> SGPLGSEAHLYMQVQIVAEDQFCGHQGNDMYDEEKVKYTVFKVLKNSSLAEFVQSLSQTMGFPQDQIRLWPMQARSNGTKRPAMLDNEADGNKTMIELSDNENPWTIFLETVDPELAASGATLPKFDKDHDVMLFLKMYDPKTRSLNYCGHIYTPISCKIRDLLPVMCDRAGFIQDTSLILYEEVKPNLTERIQDYDVSLDKALDELMDGDIIVFQKDDPENDNSELPTAKEYFRDL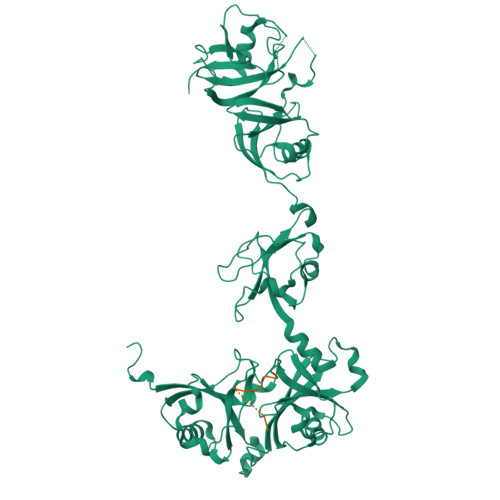YHRVDVIFCDKTIPNDPGFVVTLSNRMNYFQVAKTVAQRLNTDPMLLQFFKSQGYRDGPGNPLRHNYEGTLRDLLQFFKPRQPKKLYYQQLKMKITDFENRRSFKCIWLNSQFREEEITLYPDKHGCVRDLLEECKKAVELGEKASGKLRLLEIVSYKIIGVHQEDELLECLSPATSRTFRIEEIPLDQVDIDKENEMLVTVAHFHKEVFGTFGIPFLLRIHQGEHFREVMKRIQSLLDIQEKEFEKFKFAIVMMGRHQYINEDEYEVNLKDFEPQPGNMSHPRPWLGLDHFN;> SDWPNHARSPGNKGKGKGKGKGKPKSQACEPSE>[2x]MGSDKIHHHHHHMTFEEFKDRLFALAKKNGVEVQISFLETREFSLRLANGDLDQYTDAGKFNVEIKVLKDGKTGTFRTQVLENPEKCFEEALSNLQVKDSEEKEYFFEGGKEYREMETYVGRFEKL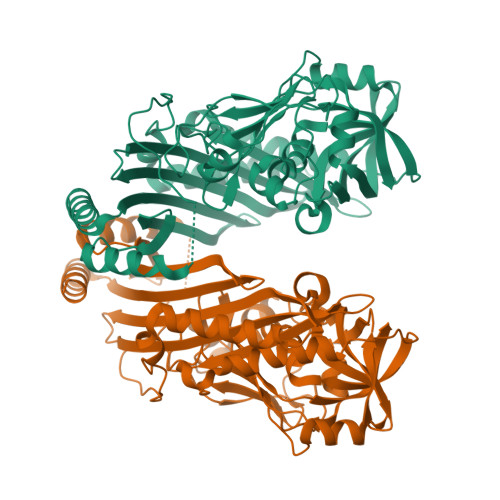SVKEKMDMAKKAHESAAKDERVVMVPTVMYKDMVIKKIITNTLGLDVESQMDGGFLFAMAIARDANPRSGSWYELARTPEDLNPEEIGKRAAEEAISLIGSKTIPSGKYPVLMRNTALLDLMEMFIPMISAENVQKNLSPLKGKLGEQVGNPAVSIKDLPYHPKGLSSTPFDDEGVPTTEKFVLENGVLKTFLHNLKTARKEGVEPTGNGFVGGIRPVNLMLMPGEKSFEELLKEMDRGVVITEVEGMHAGANSISGEFSLFAKGYWVENGEIAHGVEDITISGNFLDLLRKIVLVGNDVKVSQHTIAPSVLVEVLDVAGK> MKLLKKMMQVLLAVFFFGLLATNTVFANTTGGRFVDKDNRKYYVKDDHKAIYWHKIDGKTYYFGDIGEMVVGWQYLEIPGTGYRDNLFDNQPVNEIGLQEKWYYFGQDGALLEQTDKQVLEAKTSENTGKVYGEQYPLSAEKRTYYFDNNYAVKTGWIYEDGNWYYLNKLGNFGDDSYNPLPIGEVAKGWTQDFHVTIDIDRSKPAPWYYLDASGKMLTDWQKVNGKWYYFGSSGSMATGWKYVRGKWYYLDNKNGDMKTGWQYLGNKWYYLRSSGAMVTGWYQDGLTWYYLNAGNGDMKTGWFQVNGKWYYAYSSGALAVNTTVDGYSVNYNGEWV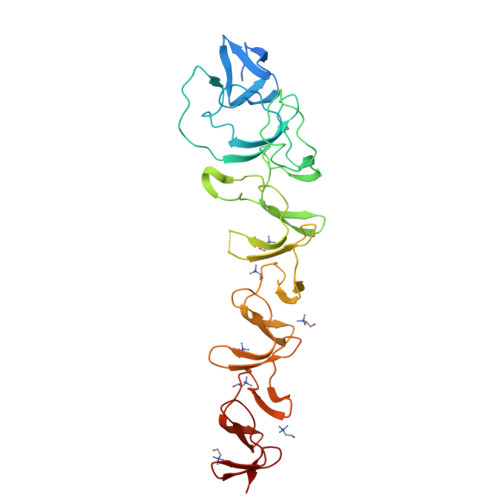Q>MRGSHHHHHHGSKLRVALSNHLLWSKFNQHQTEMIITKQGRRMFPFLSFTVAGLEPTSHYRMFVDVVLVDQHHWRYQSGKWVQCGKAEGSMPGNRLYVHPDSPN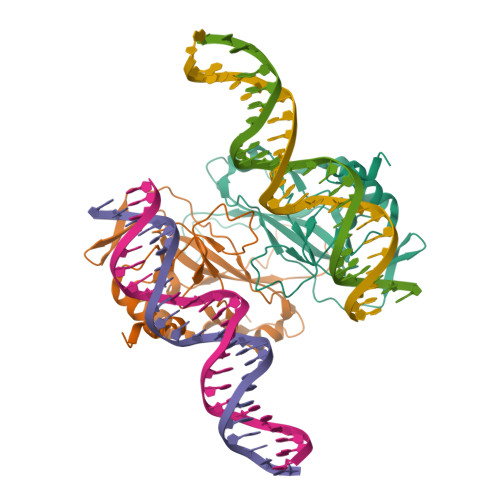TGAHWMRQEVSFGKLKLTNNKGASNNVTQMIVLQSLHKYQPRLHIVEVNDGEPEAACSASNTHVFTFQETQFIAVTAYQNAEITQLKIDNNPFAKGFREN[2x]>MSAFITFEGPEGSGKTTVINEVYHRLVKDYDVIMTREPGGVPTGEEIRKIVLEGNDMDIRTEAMLFAASRREHLVLKVIPALKEGKVVLCDRYIDSSLAYQGYARGIGVEEVRALNEFAINGLYPDLTIYLNVSAEVGRERIIKNSRDQNRLDQEDLKFHEKVIEGYQEIIHNESQRFKSVNADQPLENVVEDTYQTIIKYLEKI[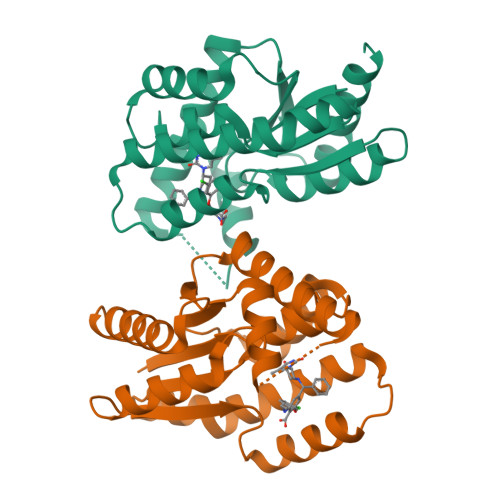2x]> MSYAVAGALQAAVYQQLRADAVLAALVGTAVYDAVPPGPLAGTYVSLGPEDVADASDKTGAGAVHDF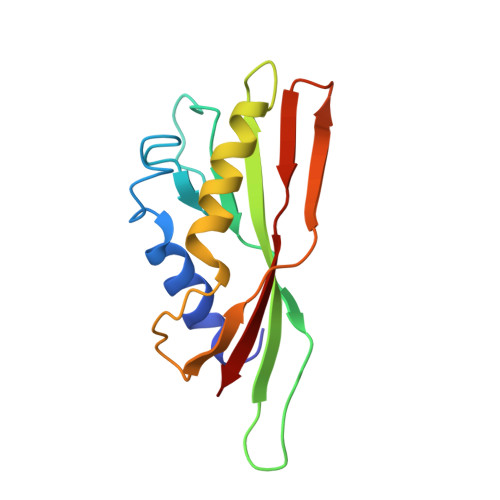VISVITDAAGFATAKAAAAAVSDALVGADLVLSRGRLVGLWFLRAKARRVEKADMRRIDLVFRARVEG> GHPVLEKLKAAHSYNPKEFEWNLKSGRVFIIKSYSEDDIHRSIKYSIWCSTEHGNKRLDSAFRCMSSKGPVYLLFSVNGSGHFCGVAEMKSPVDYGTSAGVWSQDKWKGKFDVQWIFVKDVPNNQLRHIRLENNDNKPVTNSRDTQE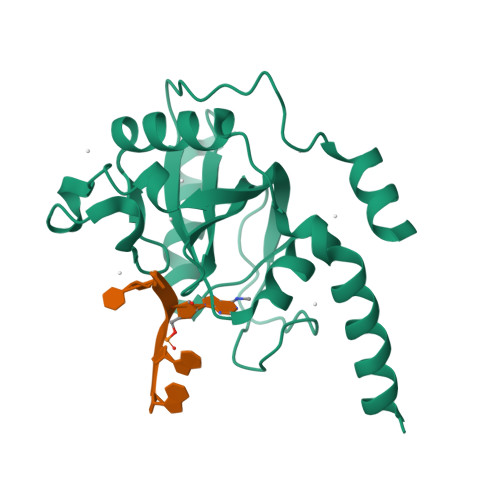VPLEKAKQVLKIISSYKHTTSIFDDFAHYEKRQEEEEVVRKERQ> MAQQSTKNETALLVAKSAKSALQDFNHDYSKSWTFGDKWDNSNTMFETFVNKYLFPKINETLLIDIALGNRFNWLAKEQDFIGQYSEEYVIMDTVPINMDLSKNEELMLKRNYPRMATKLYG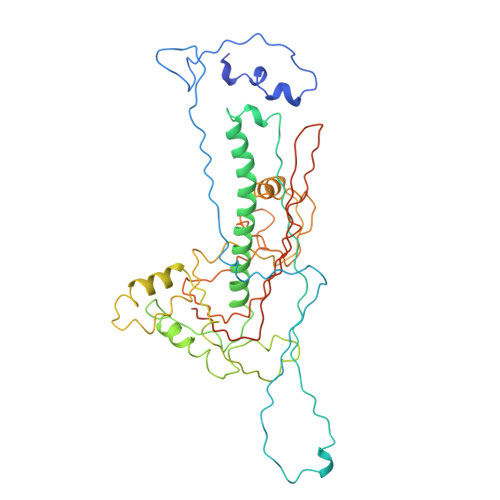NGIVKKQKFTLNNNDTRFNFQTLADATNYALGVYKKKISDINVLEEKEMRAMLVDYSLNQLSETNVRKATSKEDLASKVFEAILNLQNNSAKYNEVHRASGGAIGQYTTVSKLKDIVILTTDSLKSYLLDTKIANTFQIAGIDFTDHVISFDDLGGVFKVTKEFKLQNQDSIDFLRAYGDYQSQLGDTIPVGAVFTYDVSKLKEFTGNVEEIKPKSDLYAFILDINSIKYKRYTKGMLKPPFHNPEFDEVTHWIHYYSFKAISPFFNKILITDQDVNPKPEEELQE>MNGAIKVGAWGGNGGSAFDMGPAYRIISVKIFSGDVVDAVDVTFTYYGKTETRHFGGSGGTPHEIVLQEGEYLVGMKGEFGNYHGVVVVGKLGFSTNKKSYGPFGNTGGTPFSLPIAAGKISGFFGRGGDFIDAIG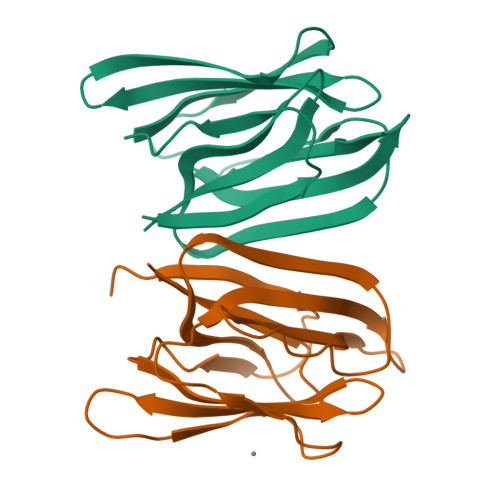VYLEP[2x]>[2x]MSFNESASIPTGLTYD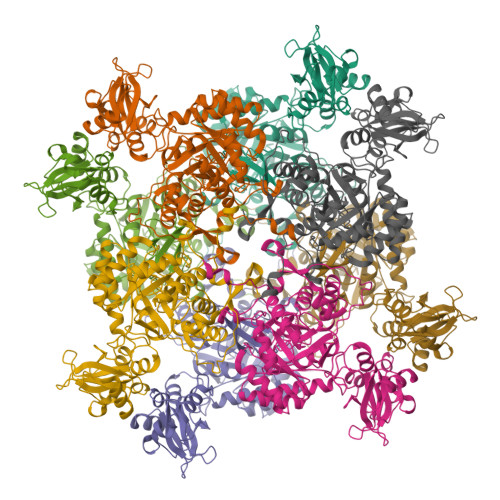DVLIIPQHSRVTSRKEVNTTTRLSRNVKLSIPIVASNMDTVCEQRMAVAMAREGGIGILHRFCSIEEQCAMLREVKRAQSFLIESPRIILPHETAREAWEGLNWKGRVGGVGCLLVVNCKNERKLLGIITRHDLKLADESTTVESLMTPVDKMVVSTNTSISLEEVTHLMRKGRTANVPIVGQNGQLLYLVTLSDVVKLRKNKQASLDSRGRLLVGAAVGVKKDDMNRAIRLVEAGADVLVVDIAHGHSDLCINMVKRLKGDPRTASVDIIAGNIASAEAAEALIDAGADGLKIGVGPGSIAITRLVAGAGVPQLSAVLACTRVARRRGVPCIADGGLRTSGDISKAIGAGADTVMLGNMLAGTDEAPGRVLVKDGQKVKIIRGMAGFGANLSKAERERTQDEDVFSSLVPEGVEGSVACKGPVGPIVRQLVGGLRSGMSYSGAKSIEEMQRRTRFVRMTGAGLRESGSHGVAKLKLAAALEHHHHHH> MEFMMEIQGNR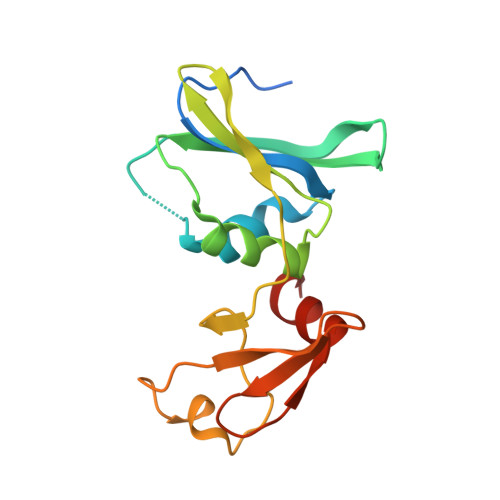KELMVSKIKNGTVIDHIPAGRAFAVLNVLGIKGHEGFRIALVINVDSKKMGKKDIVKIEDKEISDTEANLITLIAPTATINIVREYEVVKKTKLEVPKVVKGILKCPNPYCITSNDVEAIPTFKTLTEKPLKMRCEYCETIIDENEIMSQILGANNK>[2x]MKLQLALDELTLPEAMVFMDKVVDDVDIIEVGTPFLIREGVNAIKAIKEKYPHKEVLADAKIMDGGHFESQLLFDAGADYVTVLGVTDVLTIQSCIRAAKEAGKQVVVDMIC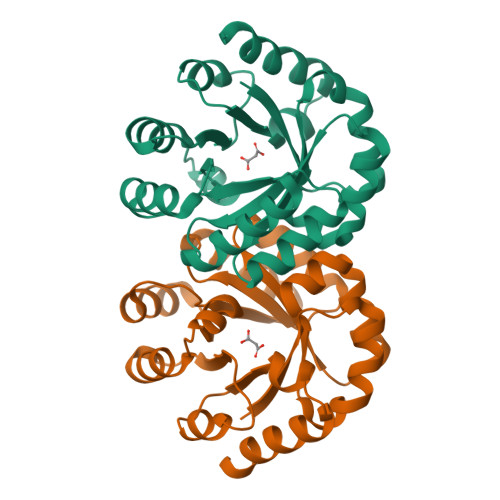VDDLPARVRLLEEAGADMLAVHTGTDQQAAGRKPIDDLITMLKVRRKARIAVAGGISSQTVKDYALLGPDVVIVGSAITHAADPAGEARKISQVLLQHH D-Mannitol-1-phosphate | C6 H15 O9 P | 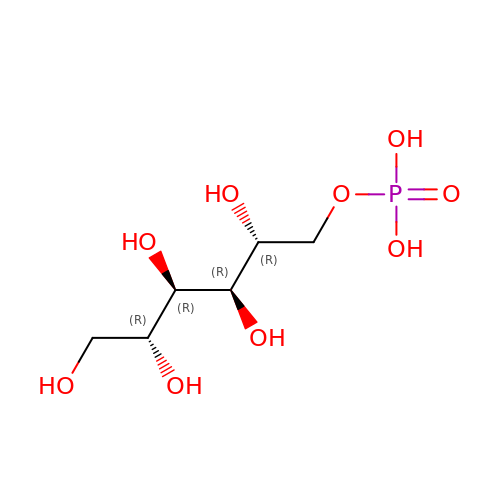GACTWZZMVMUKNG-KVTDHHQDSA-N> MKKLLPILIGLSLSGFSSLSQAENLMQVYQQARLSNPELRKSAADRDAAFEKINEARSPLLPQLGLGADYTYSNGYRDANGINSNATSASLQLTQSIFDMSKWRALTLQEKAAGIQDVTYQTDQQTLILNTATAYFNVLNAIDVLSYTQAQKEAIYRQLDQTTQRFNVGLVAITDVQNARAQYDTVLANEVTARNNLDNAVEQLRQITGNYYPELAALNVENFKTDKPQPVNALLKEAEKRNLSLLQARLSQDLAREQIRQAQDGHLPT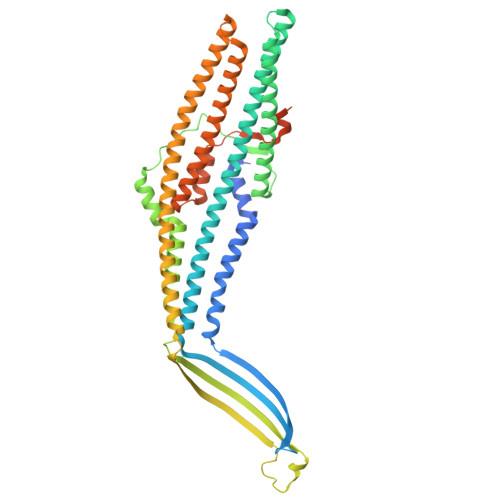LDLTASTGISDTSYSGSKTRGAAGTQYDDSNMGQNKVGLSFSLPIYQGGMVNSQVKQAQYNFVGASEQLESAHRSVVQTVRSSFNNINASISSINAYKQAVVSAQSSLDAMEAGYSVGTRTIVDVLDATTTLYNAKQELANARYNYLINQLNIKSALGTLNEQDLLALNNALSKPVSTNPENVAPQTPEQNAIADGYAPDSPAPVVQQTSARTTTSNGHNPFRN>GSHMEKRKIILDCDPGHDDAIAIMMAAKHPAIDLLGITIVAGNQTLDKTLINGLNVCQKLEINVPVYAGMPQPIMRQQIVADNIHGDTGLDGPVFEPLTRQAESTHAVKYIIDTLMASDGDITLVPVGPLSNIAVAMRMQPAILPKIREIVLMGGAYGTGNFTPSAEFNIFADPEAARVVFTSGVPLVMMGLDLTNQTVCTPDVIARMERAGGPAGELFSDIMNFTLKTQFENYGLAGGPVHDATCIGYLINPDGIKT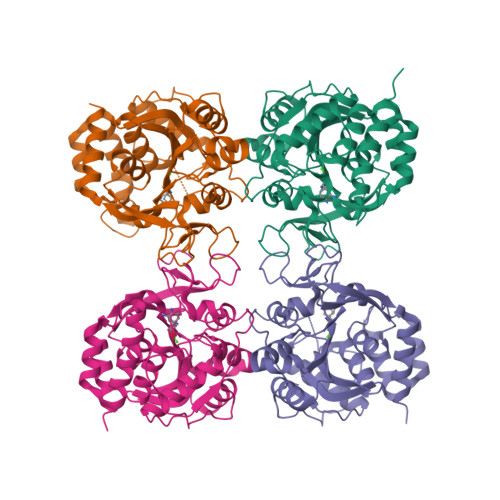QEMYVEVDVNSGPCYGRTVCDELGVLGKPANTKVGITIDTDWFWGLVEECVRGYIKTH[4x]>MAPSRKFFVGGNWKMNGRKQSLGELIGTLNAAKVPADTEVVCAPPTAYIDFARQKLDPKIAVAAQNCYKVTNGAFTGEISPGMIKDCGATWVVLGHSERRHVFGESDELIGQKVAHALAEGLGVIACIGEKLDEREAGITEKVVFEQTKVIADNMKDWS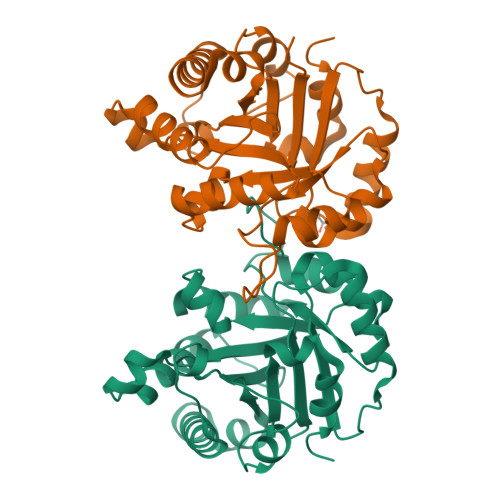KVVLAYEPVWAIGTGKTATPQQAQEVHEKLRGWLKSNVSDAVAQSTRIIYGGSVTGATCKELASQPDVDGFLVGGASLKPEFVDIINAKQ[2x]> MGLSPAFAATAGCRLASPVANSSRFLSLLRLSRPRLNAA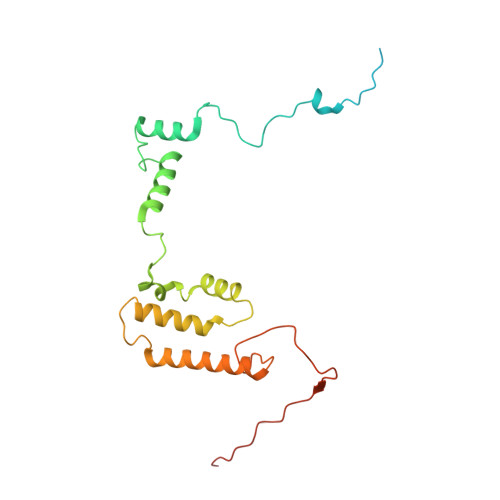APAAEAAKTLERNVPMKEILQPLWVVEPPNFLRQPVWKQFWEAQFANRSFFFFGNAWTSAAAFAFFIWWSRVFDPPPKERLDRYWLNSPKFRILSAFHNPGKRPGLKISLMTYEARYCYRGLDHPFTLNEMKDFLFKLREQYLVNKYEGIQFPFVFRQFNRVSTPGTLEVHTSPALQQQPHFHEEAAGHH> SNAMSYINNIEHAKVLDLTQEVMIEQDQMLSRTLVQRQDLGITVFSLDKGQEIGRHSSPGDAMVTILSGLAEITIDQETYRVAEGQ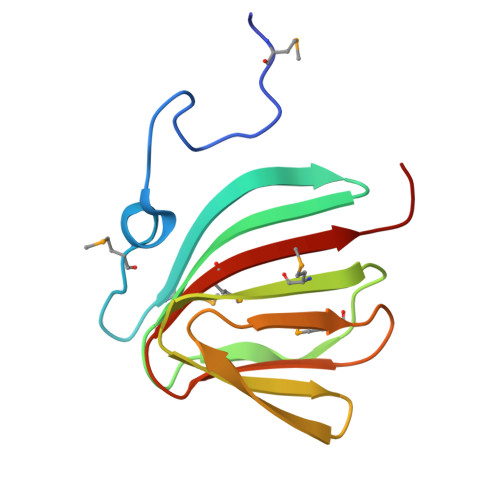TIVMPAGIPHALYAVEAFQMLLVVVKPEA>[3x]MGSSHHHHHHSAGENLYFQGTLPRETDEEPEEPGRRG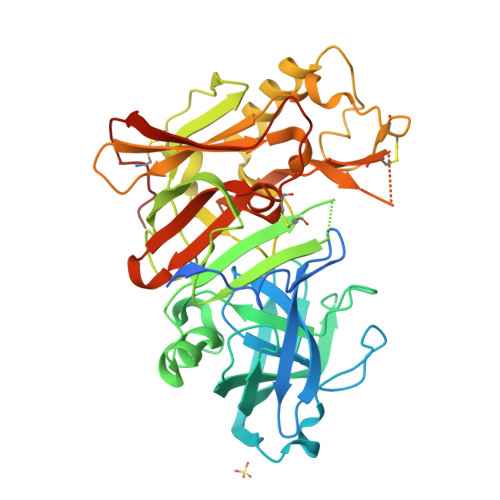SFVEMVDNLRGKSGQGYYVEMTVGSPPQTLNILVDTGSSNFAVGAAPHPFLHRYYQRQLSSTYRDLRKGVYVPYTQGAWAGELGTDLVSIPHGPNVTVRANIAAITESDKFFINGSNWEGILGLAYAEIARPDDSLEPFFDSLVKQTHVPNLFSLQLCGAGFPLNQSEVLASVGGSMIIGGIDHSLYTGSLWYTPIRREWYYEVIIVRVEINGQDLKMDCKEYNYDKSIVDSGTTNLRLPKKVFEAAVKSIKAASSTEKFPDGFWLGEQLVCWQAGTTPWNIFPVISLYLMGEVTNQSFRITILPQQYLRPVEDVATSQDDCYKFAISQSSTGTVMGAVIMEGFYVVFDRARKRIGFAVSACHVHDEFRTAAVEGPFVTLDMEDCGYNIPQTDEST(3S)-3-HYDROXYBUTANOIC ACID | 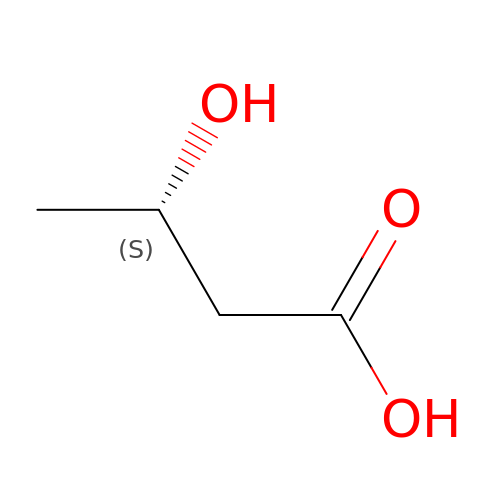C4 H8 O3 | WHBMMWSBFZVSSR-VKHMYHEASA-N>[4x]MAHHHHHHTKAEKIVAVTACPVGVAHTYIAA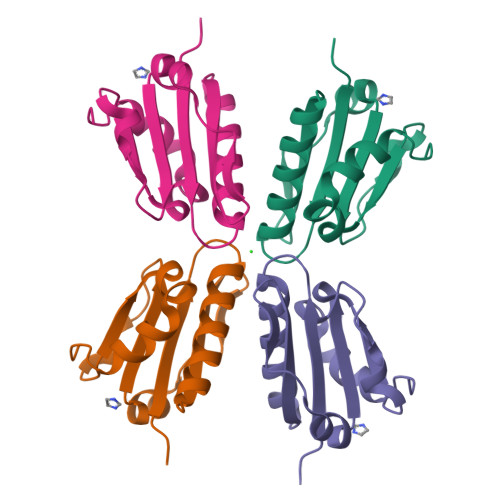KKIENEAKKQGYSIRVETQGSIGIENALTEEEIKNASVVILAVDKDIDEKRFEGKRVYKVSTVKAINNTENIIKESFNAPVF>MSDNDELQQIAHLRREYTKGGLRRRDLPADPLTLFERWLSQACEAKLADPTAMVVATVDEHGQPYQRIVLLKHYDEKGMVFYTNLGSRKAHQIENNPRVSLLFPWHTLERQVMVIGKAERLSTLEVMKYFHSRPRDSQIGAW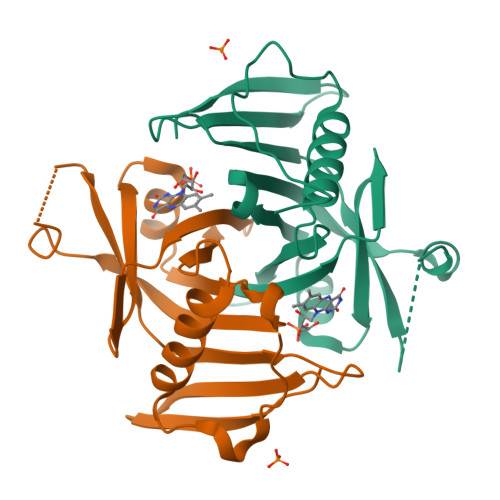VSKQSSRISARGILESKFLELKQKFQQGEVPLPSFWGGFRVSLEQIEFWQGGEHRLHDRFLYQRENDAWKIDRLAP[2x]> MSLDIQSLDIQCEELSDARWAELLPLLQQCQVVRLDDCGLTEARCKDISSALRVNPALAELNLRSNELGDVGVHCVLQGLQTPSCKIQKLSLQNCCLTGAGCGVLSSTLRTLPTLQELHLSDNLLGDAGLQLLCEGLLDPQCRLEKLQLEYCSLSAASCEPLASVLRAKPDFKELTVSNNDINEAGVRVLCQGLKDSPCQLEALKLESCGVTSDNCRDLCGIVASKASLRELALGSNKLGDVGMAELCPGLLHPSSRLRTLWIWECGITAKGCGDLCRVLRAKESLKELSLAGNELGDEGARLLCETLLEPGCQLESLWVKSCSFTAACCSHFSSVLAQNRFLLELQISN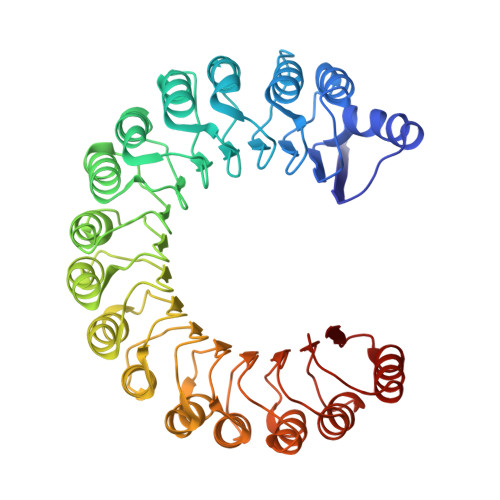NRLEDAGVRELCQGLGQPGSVLRVLWLADCDVSDSSCSSLAATLLANHSLRELDLSNNCLGDAGILQLVESVRQPGCLLEQLVLYDIYWSEEMEDRLQALEKDKPSLRVIS>MSVIKQVMKTKLHLEGTVNGHDFTIEGKGEGKPYEGLQHMKMTVTKGAPLPFSVHILTPSHMYGSKPFNKYPADIPDYHKQSFPEGMSWERSMIFEDGGVCTASNHSSINLQENCFIYDVKFHGVNLPPDGPVMQKTIAGWEPSVETLYVRDGMLKSDTAMVFKLKGGGHHRVDFKTTYKAKKPVKLPEFHFVEHRLELT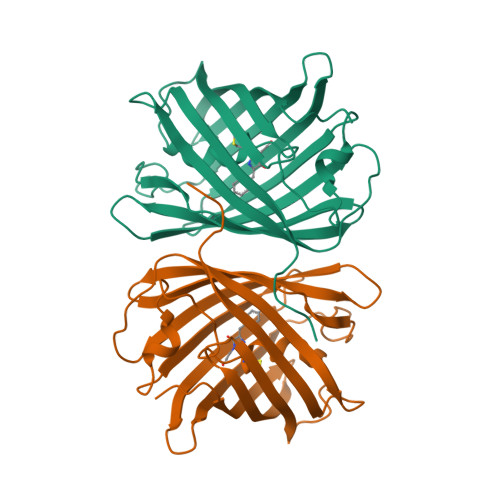KHDKDFTTWDQQEAAEGHFSPLPKALP[4x]> CSLPGLSAAADQTIKIGAQSMSESEIIASMLGQLIEHHTDLKTTTIKNLGSNAVQQQALMNGEIDIAATRYTGDALTGTLRMEPEKDPDKALALTQREFKKRYDLKWYDSYGFDNTYAFTVSKELADQYHLETVSDVKKWAPQLKLGVDNYWMKLKGNGYQDFTKTYGMTFGGTY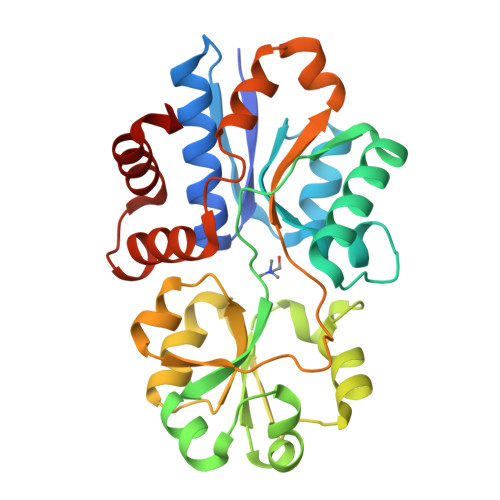PMQIGLVYDAVKSGKMDIVLAYSTDGRIKSYGLKMLKDDKQFFPPYDCSPVVPEKVLKEHPELEGIIKKMLGKIDTATMQELNYEVDGNLKEPSVVAKEYLEKHRYFES>MKDIAIRGYCDRPSVATGETIRFYVSANETRGTFDAELVRLIHGDSNPAGPGYKEEAIKSDLEGQYPARFQRTQFGSYVEVADPDAGLQPDGAFSVHLFLWSTTPSRGRQGIASRWNDERQSGWNLAIEDGRVVFTIGDGSGATSSVVSDRPLFQQIWYSITGVYDPEKKQLRLYQKSVVNRTNSRFGLVVPLDSDCAVSADATVKAADSETSLLIAGLGEAAAQDGRTWCIAHYNGKVDAPKIYGCALGQDDAEKLSRGEIVRPISRLAHWDFSAGIGLNGIPTDHVVDASGYGHHGRCMNQPSRGSTGWNWDGHEENFIHCPEQYGALWFHEDCLDDCRWEKDFEFTVPEGLKSDFYAVKIRYEDTEDYIPFFVLPPRGTATAPILVIASTLSYLAYANEQIMHKADIGQAVAGHTPVLNENDVELHKNLSYYGLSTYDGHIDGRGVQYTSWRRPIMNLRPKHRQGFGSIWELPADLHLIDWLNHNGFEYDVATEHDLNDQGAELLRRYKVVLTGSHPAYQTWANADAWEDYLADGGRGMYLAANGMYWIVEVHPEKPWVMEVRKELGVTAWEAPPGEYHYSTNGRRGGRFRGRARATQKIWGTGMSSFGFDHSGYFVQMPDSQDERVAWIMEGIDPEERIGDGGLVGGGAGGYELDRYDLALGTPPNTLLLASSVEHSVVYTVIPDDKAFPHPGMNGGEHPFVRADITYFSTANGGGMFATSSISWLGSLSWNDYDNNVSKMTKNVLNQFIKDEPAPRVKLAAALEHHHHHH[4x];>MTEASESCVRDPSNYRDRSADWYAFYDERRRKEIIDIIDEHPEIVEEHAANPFGYRKHPSPYLQRVHNYFRMQPTFGRYYIYSEREWDAYRIATIREFGELPELGDERFKTEEEAMHAVFLRRIEDVRAELA[4x]

Certain bacterial species from genera such as Paracoccus, Pseudomonas, and Alcaligenes have evolved to use DMF as a sole carbon and nitrogen source for growth via degradation by a dimethylformamidase (DMFase). We show that DMFase from Paracoccus sp. strain DMF is a halophilic and thermostable enzyme comprising a multimeric complex of the α2β2 or (α2β2)2 type. The active site consists of a mononuclear iron coordinated by two Tyr side‐chain phenolates and one carboxylate from Glu. The Fe3+ ion in the active site catalyzes the hydrolytic cleavage of the amide bond in DMF.

The mutants Y440A and E521A were catalytically inactive. Structures of these mutant enzymes determined by cryoEM show a loss of Fe atoms. In the EM structures of the active site mutants (Y440A and E521A), the interface between the large and the small subunit becomes disordered, thus suggesting a role for the small subunit in the substrate entry pathway.>MNPNQKIITIGSVCMTIGMANLILQIGNIISIWISHSIQLGNQNQIETCNQSVITYENNTWVNQTYVNISNTNFAAGQSVVSVKLAGNSSLCPVSGWAIYSKDNSVRIGSKGDVFVIREPFISCSPLECRTFFLTQGALLNDKHSNGTIKDRSPYRTLMSCPIGEVPSPYNSRFESVAWSASACHDGINWLTIGISGPDNGAVAVLKYNGIITDTIKSWRNNILRTQESECACVNGSCFTVMTDGPSNGQASYKIFRIEKGKIVKSVEMNAPNYHYEECSCYPDSSEITCVCRDNWHGSNRPWVSFNQNLEYQIGYICSGIFGDNPRPNDKTGSCGPVSSNGANGVKGFSFKYGNGVWIGRTKSISSRNGFEMIWDPNGWTGTDNNFSIKQDIVGINEWSGYSGSFVQHPELTGLDCIRPCFWVELIRGRPKENTIWTSGSSISFCGVNSDTVGWSWPDGAELPFTIDK[4x]

Stimulated by the first neuraminidase (NA) crystal structures, the NAIs were designed to interact with the active site of all NA types. We identified a novel isoleucine to arginine change at position 223 (I223R) in the NA of a virus isolated from an immune suppressed child on prolonged oseltamivir and zanamivir therapy. In contrast to the frequently observed H275Y change, which causes selective resistance to oseltamivir, the I223R mutation conferred a resistance phenotype against both oseltamivir and zanamivir. Our results support this suggestion by indicating that a ligand-free form of the pandemic neuraminidase adopts an open conformation. Together with this structure we present the structures of the I223R mutant neuraminidase in complex with oseltamivir and zanamivir to investigate the resistance mechanism of the I223R mutant neuraminidase.

Crystals of wild type and mutant neuraminidases were grown in the absence or presence of the oseltamivir and zanamivir neuraminidase inhibitors. Instead of the hydrophobic pentoxyl substituent present in oseltamivir, zanamivir possesses the same polar glycerol substituent as sialic acid. Consequently, binding of zanamivir to the active site of neuraminidase does not require the reorientation of the side chain of E277. In the case of the wild type neuraminidase, the glycerol moiety of zanamivir forms two hydrogen bonds with E277. This interaction is unaffected in the H275Y mutant.> MEKVKKIVLIGASGFVGSALLNEALNRGFEVTAVVRHPEKIKIENEHLKVKKADVSSLDEVCEVCKGADAVISAFNPGWNNPDIYDETIKVYLTIIDGVKKAGVNRFLMVGGAGSLFIAPGLRLMDSGEVPENILPGVKALGEFYLNFLMKEKEIDWVFFSPA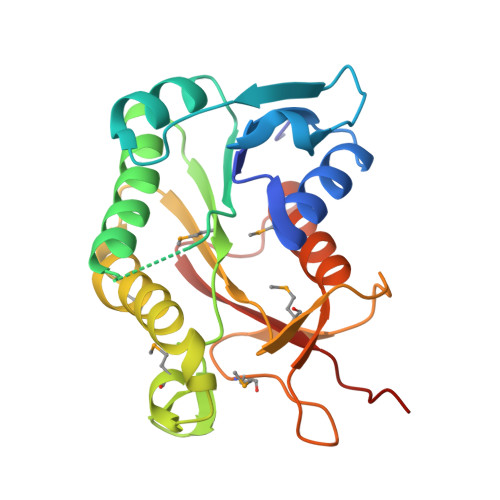ADMRPGVRTGRYRLGKDDMIVDIVGNSHISVEDYAAAMIDELEHPKHHQERFTIGYLEHHHHHH FrpD is a highly conserved lipoprotein located in the outer membrane of all meningococcal strains, and it does not exhibit similarity to known protein sequences from other organisms. Intriguingly, the FrpC1-414 fragment exhibits a very high affinity (KD ~ 0.2 nM) for FrpD, the other protein expressed from the iron-regulated frpDC operon. FrpD displays a compact, slightly concave bean-shaped structure and consists of fourteen β strands (β1–β14), one 310 helix (η1), two short α helices (α1, α2), and one long C-terminal helix α3. Hence, the similarity of FrpD fold topology to other proteins was not sufficient for establishment of structural homology, indicating that FrpD possesses a novel fold.

The FrpD43-271 protein (FrpD), a construct lacking the first 42 residues encompassing the N-terminal signal peptide (residues 1–24) and the linker sequence (residues 24–43), has been previously characterized. The protein crystallized in two alternative crystal forms, belonging to the hexagonal space group P64 and the orthorhombic space group P212121, both accommodating a single molecule in the asymmetric unit. Experimental phases were obtained from single-wavelength anomalous dispersion (SAD) of crystals of selenomethionine-labelled FrpD protein (SeMet FrpD) grown in the orthorhombic space group. The structure of the SeMet FrpD protein was refined to 1.4 Å resolution with an R value of 16.8% (Rfree of 19.3%). Here, we determined the crystal structure of the FrpD43-271 at 1.4 Å resolution. The refined crystallographic models of FrpD comprise 224 of the 229 residues, with one N-terminal and four C-terminal residues being disordered. Both FrpD structures are largely identical, with a coordinate root-mean-square deviation (rmsd) of 0.56 Å over the 224 aligned residues. The structure is characterized by a C-terminal α-helix (α3) that traverses a series of antiparallel β-strands. A single disulphide bond in a right-handed spiral conformation is present between the Cys150 and Cys227 residues. The electrostatic surface potential map revealed that the FrpD surface is highly negatively charged, except for a single positively charged region located at the β9 and β10 strands of the structure.

> KEQTSFNNPEPMTGFEHTVTFDFQGTKMVIPYGYLARYTQDNATKWLSDTPGQDAYSINLIEISVYYKKTDQGWVLEPYNQQNKAHFIQFLRDGLDSVDDIVIRKDACSLSTTMGERLLTYGVKKMPSAYPEYEAYEDKRHIPENPYFHEFYYIKKGENPAIITHRNNRINQTEEDSYSTSVGSCINGFTVQYYPFIREKQQLTQQELVGYHQQVEQLVQSFVNNSNKKENLYFQGLEHHHHHH> ENSLEIEELARFAVDEHNKKENALLEFVRVV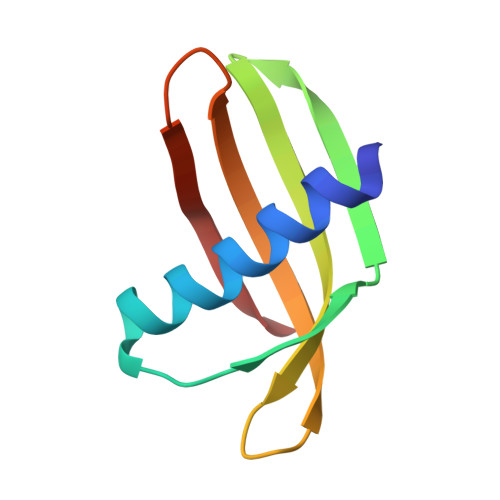KAKEQVVAGTMYYLTLEAKDGGKKKLYEAKVWVKPWENFKELQEFKPV> MRGSHHHHHHGLVPRGSMIRTMLQGKLHRVKVTHADLHYEG;> MKLTIIRLEKFSDQDRIDLQKIWPEYSPSSLQVDDNHRIYAARFNERLLAAVRVTLSGTEGALDSLRVREVTRRRGVGQYLLEEVLRNNPGVSCWWMADAGVEDRGVMTAFMQALGFTAQQGGWEKCSGLEHHHHHH;> XCAIDQDFLDAAGILENEAIDIWNVTNGKRFSTYAIAAERGSRIISVNGAAAHCASVGDIVIIASFVTMPDEEARTWRPNV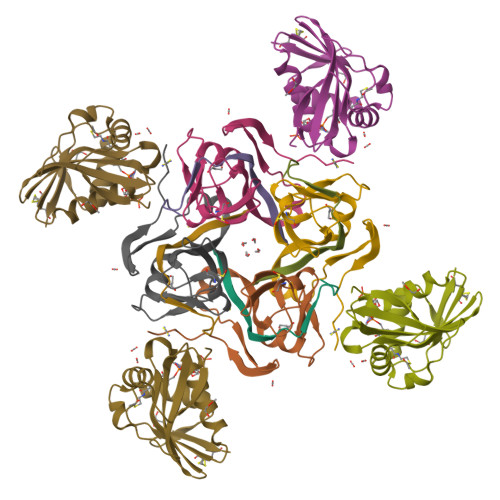AYFEGDNEMKRTAKAIPVQVA>MSLTEKFRPTLKDVARQAGVSIATASRALADNPAVAASTRERIQQLASDLGYRANAQARALRSSRSNTIGVIVPSLINHYFAAMVTEIQSTASKAGLATIITNSNEDATTMSGSLE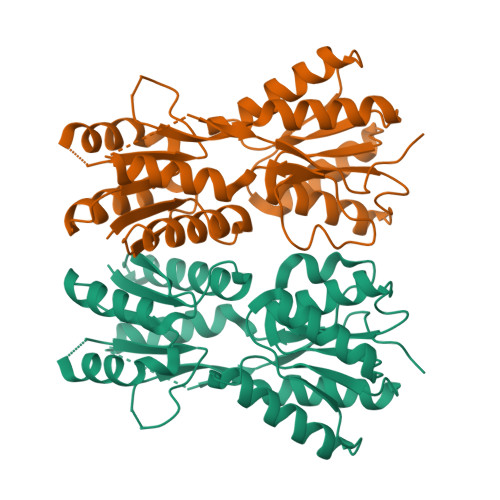FLTSHGVDGIICVPNEECANQLEDLQKQGMPVVLVDRELPGDSTIPTATSNPQPGIAAAVELLAHNNALPIGYLSGPMDTSTGRERLEDFKAACANSKIGEQLVFLGGYEQSVGFEGATKLLDQGAKTLFAGDSMMTIGVIEACHKAGLVIGKDVSVIGFDTHPLFALQPHPLTVIDQNVEQLAQRAVSILTELIAGTVPSVTKTTIPTALIHRESIINSTLRKEGHHHHHH[2x]> MASVDFKTYVDQACRAAEEFVNVYYTTMDKRRRLLSRLYMGTATLVWNGNAVSGQESLSEFFEMLPSSEFQISVVDCQPVHDEATPSQTTVLVVICGSVKFEGNKQRDFNQNFILTAQASPSNTVWKIASDC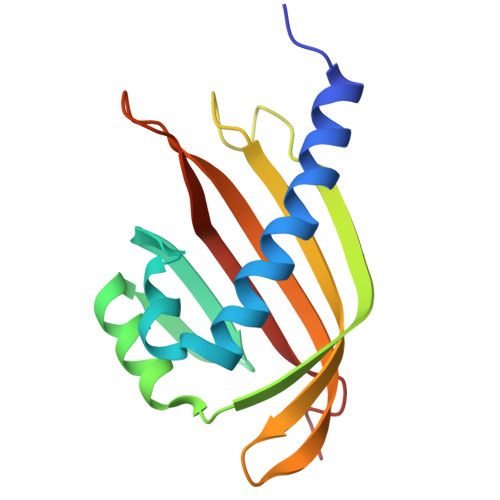FRFQDWAS> APRKARTAF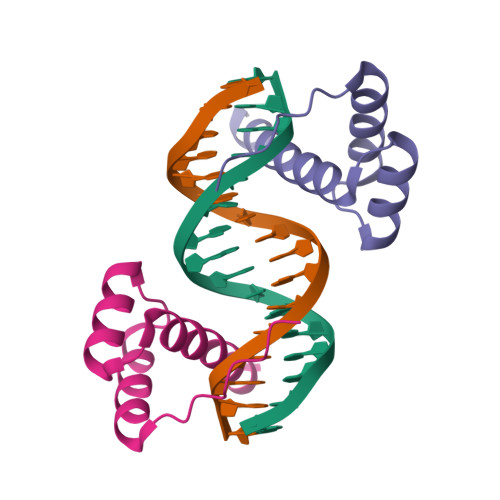SDHQLNQLERSFERQKYLSVQDRMDLAAALNLTDTQVKTWYQNRRTKWKRQTAVG;> KKPRKARTAFSDHQLNQLERSFERQKYLSVQDRMDLAAALNLTDTQVKTWYQNRRTKWKRQTA> LGTNYLLSGQTLETEGHLKNGDFDLVMQDDCNLVLYNGNWQSNTANKGRDCKLTLTDYGELVINNGDGSTVWRSKAQSVKGDYAAVDHPEGRLVVFGPSVFKIDPWVPG;> NIPFTNNLLFSGQVLYGDGRLTAKNHQLVMQGDCNLVLYGGKYGWQSNTHGNGEHCFLRLNHKGELIIKD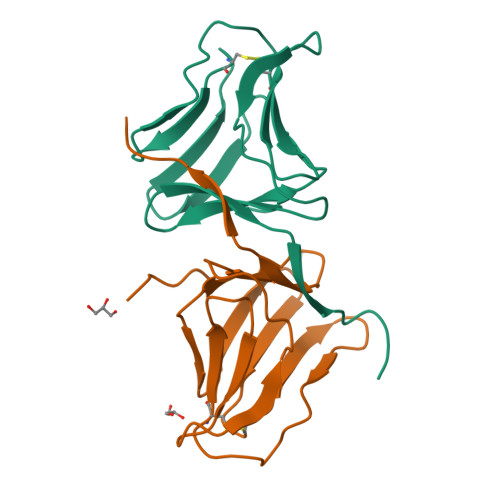DDFKTIWSSSSSSKQGDYVLILRDDGFAVIYGPAIWETSPQ>ENLYFQSDDHFGLHGLVFRRTFAIRSYEVGPDRSTSILAVMNHMQEATLNHAKSVGILGDGFGTTLEMSKRDLMWVVRRTHVAVERYPTWGDTVEVECWIGASGNNGMRRDFLVRDCKTGEILTRCTSLSVLMNTRTRRLSTIPDEVRGEIGPAFIDNVAVKDDEIKKLQKLNDSTADYIQGGLTPRWNDLDVNQHVNNLKYVAWVFETVPDSIFESHHISSFTLEYRRECTRDSVLRSLTTVSGGSSEAGLVCDHLLQLEGGSE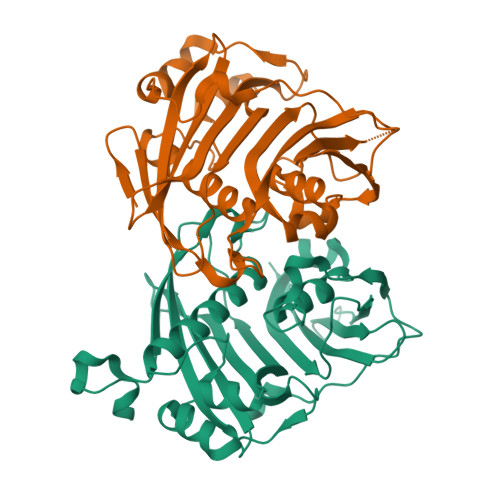VLRARTEWRPK[2x]> MESYHKPDQQKLQALKDTANRLRISSIQATTAAGSGHPTSCCSAAEIMAVLFFHTMRYKSQDPRNPHNDRFVLSKGHAAPILYAVWAEAGFLAEAELLNLRKISSDLDGHPVPKQAFTDVATGSLGQGLGAACGMAYTGKYFDKASYRVYCLLGDGELSEGSVWEAMAFASIYKLDNLVAILDINRLGQSDPAPLQHQMDIYQKRCEAFGWHAIIVDGHSVEELCKAFGQAKHQPTAIIAKTFKGRGITGVEDKESWHGKPLPKNMAEQIIQEIYSQIQSKKKILATPPQEDAPSVDIANIRMPSLPSYKVGDKIATRKAYGQALAKLGHASDRIIALDGDTKNSTFSEIFKKEHPDRFIECYIAEQNMVSIAVGCATRNRTVPFCSTFAAFFTRAFDQIRMAAISESNINLCGSHCGVSIGEDGPSQMALEDLAMFRSVPTSTVFYPSDGVATEKAVELAANTKGICFIRTSRPENAIIYNNNEDFQVGQAKVVLKSKDDQVTVIGAGVTLHEALAAAELLKKEKINIRVLDPFTIKPLDRKLILD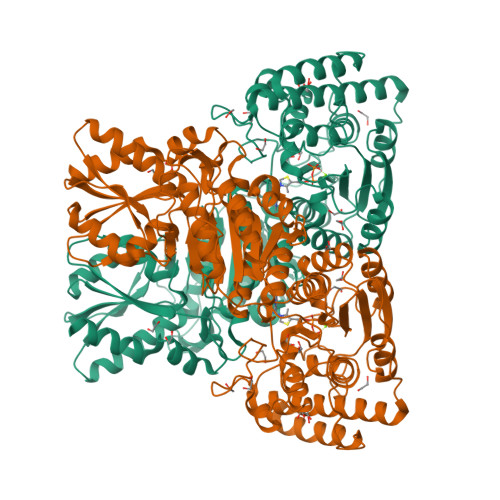SARATKGRILTVEDHYYEGGIGEAVSSAVVGEPGITVTHLAVNRVPRSGKPAELLKMFGIDRDAIAQAVRGLITKALVPRGSLEHHHHHH>LTLGNTTSSVILTNYMDTQYYGEIGIGTPPQTFKVVFDTGSSNVWVPSSKCSRLYTACVYHKLFDASDSSSYKHNGTELTLRYSTGTVSGFLSQDIITVGGITVTQMFGEVTEMPALPFMLAEFDGVVGMGFIEQAIGRVTPIFDNIISQGVLKEDVFSFYYNRDSENSQSLGGQIVLGGSDPQHYEGNFHYINLIKTGVWQIQMKGVSVGSSTLLCEDGCLALVDTGASYISGSTSSIEKLMEALGAKKRLFDYVVKCNEGPTLPDISFHLGGKEYTLTSADYVFQESYSSKKLCTL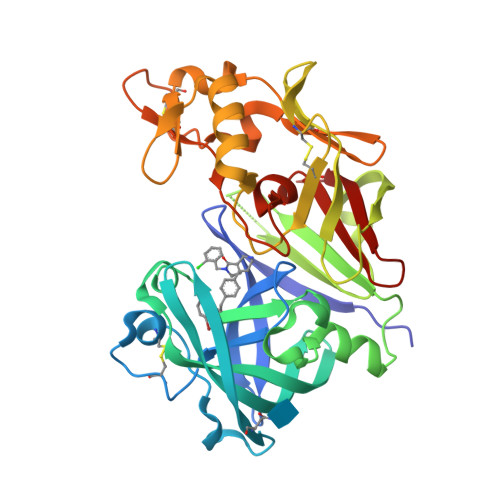AIHAMDIPPPTGPTWALGATFIRKFYTEFDRRNNRIGFALARH[2x]> GAMGSGIQMKEEASEHGGSADETQELSPVSDSSDEMPNNAKRRRRSQSMIANKRIHQAFQEDEGDEDWEEEEHKPKAKRRYNTRSNESFSEGDDEPFEVSESSALEDELSDSEDSFIRSVRSKPKYKPGTRRSTRLRNRRSQDEEESEEEHRPILRERTSRINYSVPLAFPPVDEMDGDPSSQVNQSRSRKTHSELAITKLLRQQVSSFMPYIDSSGSESESDNTRIKKSSAKTIKALTDPANSGGPPDFGRIREKSDLADSDPLGVDSSLSFESVGGLDNYINQLKEMVMLPLLYPEIFQRFNMQPPRGVLFHGPPGTGKTLMARALAAACSSENKKVSFYMRKGADCLSKWVGEAERQLRLLFEEAKSTQPSIIFFDQIDGLAPVRSSKQEQIHASIVSTLLALMDGMESRGQVIIIGATNRPDAVDPALRRPGRFDREFYFPLPDRDARKKIIEIHTRNWDPPVPEWLCSMLAEKSKGYGGADLRALCTEAALNSIKRTYPQLYRSTKRLQIDPKTIKVKVKDFVMSMKRMIPSSERSSISPSKPLSPELKPLLNEAFQDIEKTLQKLMPVASKLNPLEEVMYDDPKENDFEYQQRLETFETLRIYKPRFLICGRKGLGQTALGPAILQQYEGVHVQSFDMSTLLQDSTQSIETSIIHLFLEVRRHTPSIIYIPDIDNWLNVLPLTAITTFSSMLERLDFSDQILFLALSSSPLSELHPQLREWFSSKQSVYSLQYPTRDSIIAFFQPILELIKASPTELPGGIPRKRRVLPELPLAPDPPPFTSQKITLKQTKQADMRLLNKLKIKLNALLGSLRARYRKFKKPLIDFNDIYCVDPETGHSYRSREECHYEFVDDVVKQIGSDQKFSMMSLEEIEKRTWDNCYCTPKQFVHDIKLILRDALQLEDSETIKRAQEMYANVLLGVEDMEDDQFSQRCERMALREAERRKLRHGKLQKHLDETKADMQFTSEKPSVDESITEVDDAIKDGPPVLAETLTNSLMEDVGPENVDMDIEDNEIFTNQSTMSVPS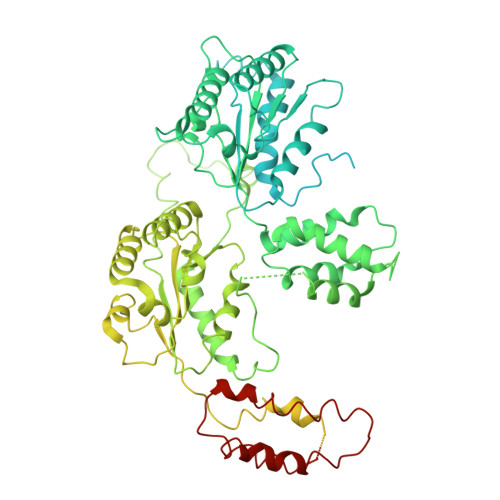MLVENEESPKPDEYIDQKDKVQSPLLNGKSPVGVPSEAALRVSTDVSTNISSNGRADIPVDTLITSPADVPNNAPTDAHNITSADGHIENIEQEVVFPDLVFDEDRLTPLKQLLIDSTTGFTVDQLLHLHSFLYQIIWNTKSEWNRNSVVDECERAVKEFMINALQ The genomes of Bacteroidales contain genes encoding glycan-degrading apparatuses that typically co-localize in discrete clusters known as polysaccharide utilization loci (PULs). B. thetaiotaomicron contains almost 300 different GHs belonging to 60 different GH families, and secretes at least six mannosyl-glycoprotein endo-β-N-acetylglucosaminidases (ENGases, endoglycosidase hereafter) that hydrolyze the chitobiose core of asparagine-linked, or N-linked, glycans (EC 3.2.1.96). Here, we discover an ENGase from the GH18 family in B. thetaiotaomicron, BT1285, encoded in a distinct PUL with its own repertoire of proteins for catabolism of the same HM N-glycan substrate as that of BT3987. Altogether, our data suggest that human gut microbes employ evolutionary strategies to express distinct ENGases in order to optimally metabolize the same N-glycan substrate in the gastroinstestinal tract.

BT1285 displays the typical (β/α)8-barrel catalytic domain found in other GH18 family members. BT1285 is a 30 kDa enzyme composed of a single GH18 catalytic domain with a TIM barrel fold typical of ENGases, while BT3987 contains an additional β-sandwich domain in the N-terminal region (DUF1735). BT1285 and BT3987 share less than 30% sequence identity and populate distinct clusters in our SSN data, accompanied by an RMSD of 2.4 Å between both ENGases, indicative of structural divergence and suggestive of the functional differences that we observe here. The main structural differences between BT1285 and BT3987 involve the length of the β-strands of the TIM barrel (particularly the β2 strand) and the presence of longer flexible loops in BT1285, with higher B-factor values around active site in BT1285 relative to those in BT3987, which decreased in the presence of the HM substrate. The overall architecture around the active site and substrate binding pocket exhibit an RMSD of 2.4 Å between these HM-processing ENGases. We identified two aromatic residues surrounding the catalytic residues that are interchanged between the two B. thetaiotaomicron HM-ENGases—Tyr315 in BT3987 is in the analogous position as Trp164 in BT1285, while Trp355 in BT3987 is in the analogous position as Tyr201 in BT1285. BT1285 exhibits significantly higher affinity and faster hydrolysis of poorly accessible HM N-glycans than does BT3987.

> MPVNQSDNNQSEVVTRSATGIKNIVYIEVNDINPLNAGSYIMDDAPFFDYVILFAANIRGVGSDATLYNNPNVQYILDHKDTLIKPLQDKGIKVLLGLLGDHTGLGFANMNSAQTEQFATAVANAVSQYGLDGVDFDDEWAEYGRNGYPSGSTGSFSNLITALHNKMPGKTITVFNYGYTSELTGVNSYIDYGIYAFFNSPSWSTGFGMPNSKFAPYTINLNSAPSAASAQLYSGQVASKGYGAIGYYDLRANNIVSVLNGVAKGAFKSTCTYDGNSYPKNY> MNDDRETPPKRKPGEDDTLFDIDFLDDTTSHSGSRSKVTNSHANANYIPPSHVLPEETIDLDADDDNIENDVHENLFMSNNHDDQTSWNANRFDSDAYQPQSLRAVKPPGLFARFGNGLKNAFTFKRKKGPESFEMNHYNAVTNNELDDNYLDSRNKFNIKILFNRYILRKNVGDAEGNGEPRVIHINDSLANSSFGYSDNHISTTKYNFATFLPKFLFQEFSKYANLFFLCTSAIQQVPHVSPTNRYTTIGTLLVVLIVSAMKECIEDIKRANSDKELNNSTAEIFSEAHDDFVEKRWIDIRVGDIIRVKSEEPIPADTIILSSSEPEGLCYIETANLDGETNLKIKQSRVETAKFIDVKTLKNMNGKVVSEQPNSSLYTYEGTMTLNDRQIPLSPDQMILRGATLRNTAWIFGLVIFTGHETKLLRNATATPIKRTAVEKIINRQIIALFTVLIVLILISSIGNVIMSTADAKHLSYLYLEGTNKAGLFFKDFLTFWILFSNLVPISLFVTVELIKYYQAFMIGSDLDLYYEKTDTPTVVRTSSLVEELGQIEYIFSDKTGTLTRNIMEFKSCSIAGHCYIDKIPEDKTATVEDGIEVGYRKFDDLKKKLNDPSDEDSPIINDFLTLLATCHTVIPEFQSDGSIKYQAASPDEGALVQGGADLGYKFIIRKPNSVTVLLEETGEEKEYQLLNICEFNSTRKRMSAIFRFPDGSIKLFCKGADTVILERLDDEANQYVEATMRHLEDYASEGLRTLCLAMRDISEGEYEEWNSIYNEAATTLDNRAEKLDEAANLIEKNLILIGATAIEDKLQDGVPETIHTLQEAGIKIWVLTGDRQETAINIGMSCRLLSEDMNLLIINEETRDDTERNLLEKINALNEHQLSTHDMNTLALVIDGKSLGFALEPELEDYLLTVAKLCKAVICCRVSPLQKALVVKMVKRKSSSLLLAIGDGANDVSMIQAAHVGVGISGMEGMQAARSADIAVGQFKFLKKLLLVHGSWSYQRISVAILYSFYKNTALYMTQFWYVFANAFSGQSIMESWTMSFYNLFFTVWPPFVIGVFDQFVSSRLLERYPQLYKLGQKGQFFSVYIFWGWIINGFFHSAIVFIGTILIYRYGFALNMHGELADHWSWGVTVYTTSVIIVLGKAALVTNQWTKFTLIAIPGSLLFWLIFFPIYASIFPHANISREYYGVVKHTYGSGVFWLTLIVLPIFALVRDFLWKYYKRMYEPETYHVIQEMQKYNISDSRPHVQQFQNAIRKVRQVQRMKKQRGFAFSQAEEGGQEKIVRMYDTTQKRGKYGELQDASANPFNDNNGLGSNDFESAEPFIENPFADGNQNSNRFSSSRDDISFDIGGGGLVPRG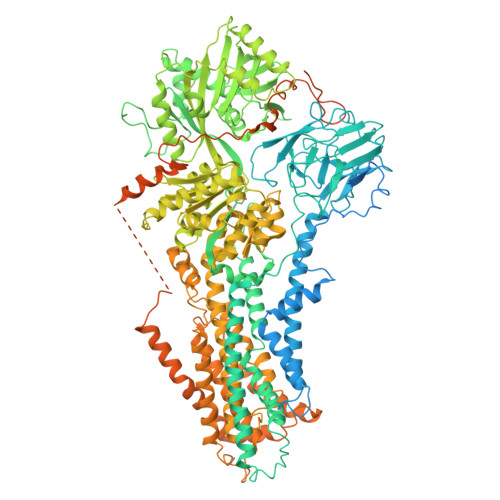SGGTAAAPGPAPAPAPASAPAAAAPAGAGTPVTAPLAGTIWKVLASEGQTVAAGEVLLILEAMKMETEIRAAQAGTVRGIAVKAGDAVAVGDTLMT> DPDSEAKKLLGLGQKHLVMGDIPAAVNAFQEAASLLGKKYGETANECGEAFFFYGKSLLELARMENGVLGNALEGVHVEEEEGEKTEDESLVENNDNIDETEGSEEDDKENDKTEEMPNDSVLENKSLQENEEEEIGNLELAWDMLDLAKIIFKRQETKEAQLYAAQAHLKLGEVSVESENYVQAVEEFQSCLNLQEQYLEAHDRLLAETHYQLGLAYGYNSQYDEAVAQFSKSIEVIENRMAVLNEQVKEAEGSSAEY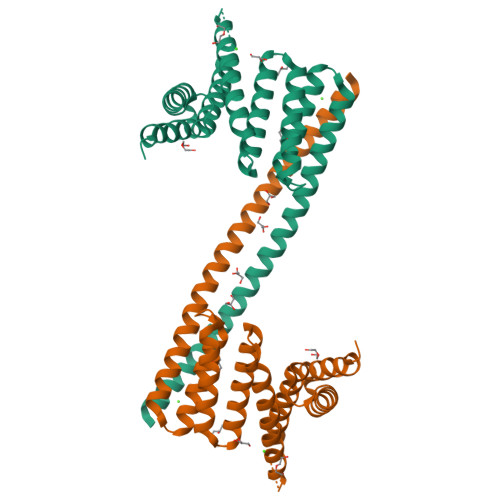KKEIEELKELLPEIREKIEDAKES> EPASTLEGPSRPVTVPLREDRGHAVDLPDTDPRVQRRVTGWAPEQIAVALSAAPTSAWVSWITGDFQMGGAVKPLDPGTVGSVVRYGLAADSLVREATGDALVYSQLYPFEGLQNYTSGIIHHVRLQGLEPGTKYYYQCGDPSIPGAMSAVHAFRTMPAVGPRSYPGRIAVVGDLGLTYNTTSTVEHMASNQPDLVLLLGDVSYANLYLTNGTGTDCYSCSFAKSTPIAETYQPRWDYWGRYMEPVTSSTPMMVVEGNHEIEQQIGNKTFAAYSARFAFPSMESESFSPFYYSFDAGGIHFIMLAAYADYSKSGEQYRWLEKDLAKVDRSVTPWLVAGWHAPWYSTYKAHYREAECMRVAMEELLYSYGLDIVFTGHVHAYERSNRVFNYTLDPCGAVHISVGDGGNREKMATTHADDPGRCPEPMSTPDAFMGGFCAFNFTSGPAAGSFCWDRQPDYSAYRESSFGHGILEVKNETHALWKWHRNQDLYQGAVGDEIYIVREPERCLLKHHHHHH

PAPs that can hydrolyze phytate are known as PAPhy (Dionisio et al., 2011). Here we show the X-ray crystal structure of the b2 isoform of wheat PAPhy induced during germination. In keeping with other HMW PAPs, TAPhy_b2 consists of a smaller fibronectin type III (FN3) non-catalytic N-terminal domain (residues Pro43–Thr156) together with a larger C-terminal MPE domain (residues Arg168–Glu497). The high-resolution crystal structures of the wheat purple acid phytase isoform b2 reported herein provide a straightforward explanation by highlighting the roles of two sequence inserts (PAPhy motifs) relative to a canonical MPE domain in forming phytate-specific substrate specificity pockets.

To validate our assignment of specificity pocket contents in TaPAPhy_b2, we turned to site-directed mutagenesis of predicted active site residues. Basic residues were chosen for alanine mutagenesis if they were found less than 6 Å from the predicted position of the bound substrate and were conserved in PAPhy but not in the non-phytase HMW PAPs. This process identified two residues highlighted from analysis of the MD trajectory, His229 (Pocket F) and Lys410 (pockets B and C), and one other, K348. The relative phytase activities of the mutants were <5% for H229A and 13% for K410A. On the other hand, the H229A mutant showed highly attenuated activity toward phytate. Crystallization of this mutant allowed its structure to be solved at 1.50 Å resolution, which proved it to be essentially identical to that of the wild-type enzyme. However, a region of discontinuous electron density was identified between residues Asp216 and Pro227, covering most of the PAPhy 4 motif. The lack of structural order in this region of the mutant enzyme can be explained by the deletion of a π-stacking interaction between His229 and Tyr218 following mutagenesis. Such interruption presumably results in instability of the PAPhy 4 motif, emphasizing the importance of this motif in phytate binding and recognition.>[6x]MPKIYTKTGDK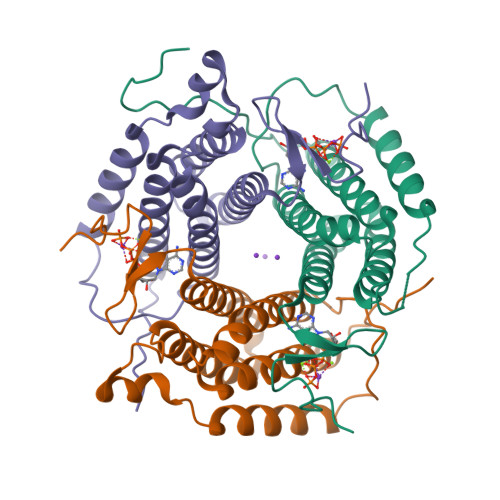GFSSTFTGERRPKDDQVFEAVGTTDELSSAIGFALELVTEKGHTFAEELQKIQCTLQDVGSALATPCSSAREAHLKYTTFKAGPILELEQWIDKYTSQLPPLTAFILPSGGKISSALHFCRAVCCRAERRVVPLVQMGETDANVAKFLNRLSDYLFTLARYAAMKEGNQEKIYMKNDPSAESEGL> GGACAUAUAAUCGCGUGGAUAUGGCACGCAAGUUUCUACCGGGCACCGUAAAUGU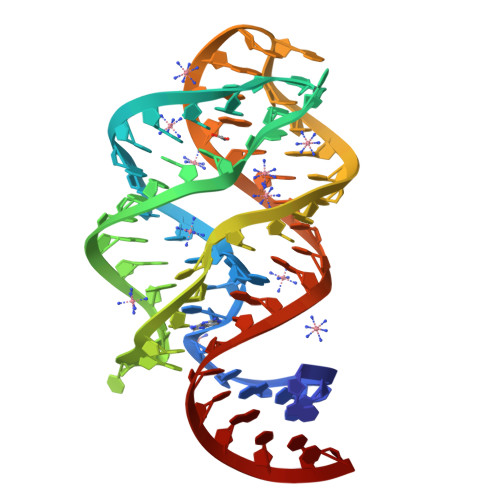CCGACUAUGUCC> MPLSQKQIDQVRTKVHYSEVDTPFNKYLDILGKVTKLTGSIINGTLSNDDSKIEKLTEQNISQLKESAHLRFLDLQSSIDTKKVADENWETCQQETLAKLENLKDKLPDIKSIHSKLLLRIGKLQGLYDSVQVINREVEGLSEGRTSLVVTRAEWEKELGTDLVKFLIEKNYLKLVDPGLKKDSSEERYRIYDDFSKGPKELESINASMKSDIENVRQEVSSYKEKWLRDAEIFGKITSIFKEELLKRDGLLNEAEGDNIDEDYESDEDEERKERFKRQRSMVEVNTIENVDEKEESDHEYDDQEDEENEEEDDMEVDVEDIKEDNEVD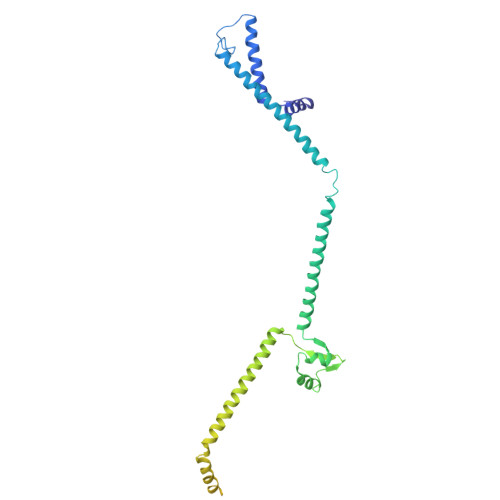GESSQQEDNSRQGNNEETDKETGVIEEPDAVNDAEEADSDHSSRKLGGTTSDFSASSSVEEVK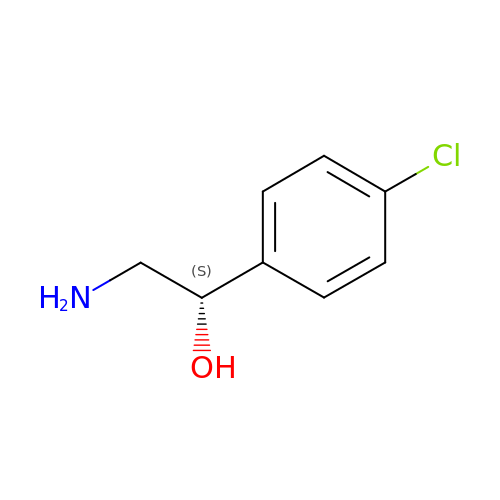(1S)-2-amino-1-(4-chlorophenyl)ethan-1-ol | C8 H10 Cl N O | QPHAZZJNYDEVHL-MRVPVSSYSA-N> NYFQGHMMQIDSIEIGGKVYQFFKSDLGNAPLLFIKGSKGYAMCGYLNM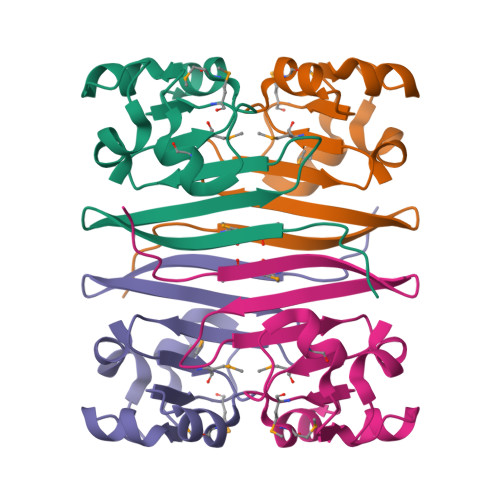ETSNKVGDIAVRVMGVKTLDDMLSAKVVEASQEAQKVGINPGDVLRNVIDKLG>[4x]GSHMSVIK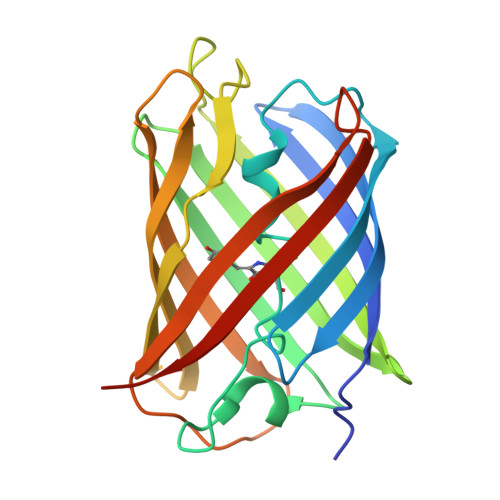PDMKIKLRMEGAVNGHPFAIEGVGLGKPFEGKQSMDLKVKEGGPLPFAYDILTTVFCYGNRVFAKYPENIVDYFKQSFPEGYSWERSMNYEDGGICNATNDITLDGDCYIYEIRFDGVNFPANGPVMQKRTVKWEPSTEKLYVRDGVLKGDVNMALSLEGGGHYRCDFKTTYKAKKVVQLPDYHFVDHHIEIKSHDKDYSNVNLHEHAEAHSELPRQAK>[7x]GPLGSPNSQARPT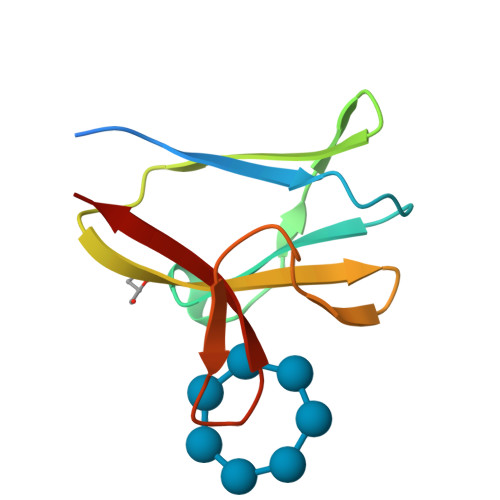VFRWTGGGKEVYLSGSFNNWSKLPLTRSQNNFVAILDLPEGEHQYKFFVDGQWTHDPSEPIVTSQLGTVNNIIQVK>GPGSELPQMVQQLNSPDQQELQSALRKLSQIASGGNEQIQAVIDAGALPALVQLLSSPNEQILQEALWTLGNIASGGNEQIQAVIDAGALPALVQLLSSPNEQILQEALWTLGNIASGGNEQIQAVIDAGALPALVQLLSSPNEQILQEALWTLGNIASGGNEQIQAVIDAGALPALVQLLSSPNEQILQEALWTLGNIASGGNEQIQAVIDAGALPALVQLLSSPNEQILQEALWTLGNIASGGNEQIQAVIDAGALPALVQLLSSPNEQILQEALWTLGNI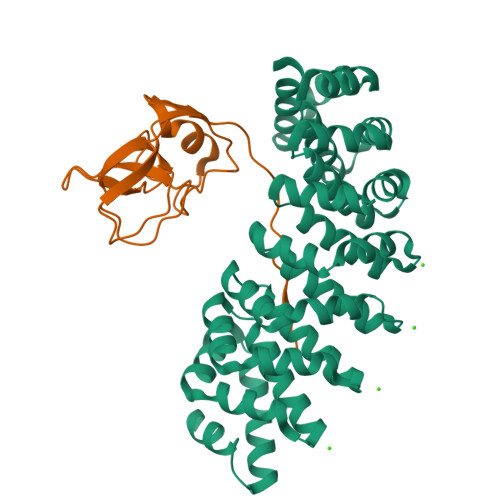ASGGNEQKQAVKEAGALEKLEQLQSHENEKIQKEAQEALEKLQSH[8x];>GPTATAPGGLSAKAPAMTPLMLDTSSRKLVAWDGTTDGAAVGILAVAADQTSTTLTFYKSGTFRYEDVLWPEAASDETKKRTAFAGTAISIVGSGSPKRKRKRKRKREG[4x]> GATGRTTIAIDPVTRIEGHLKAEVVVENGKVVDARLSGGMYRGFETILRGRDPRDASQIVQRICGVCPTAHSTASVLALDEAFGAKVPNNGRITRNLIFGANYLQSHILHFYHLSAQDFVQGPDTAPFVPRFPKSDLRLSKELNKAGVDQYIEALEVRRICHEMVALFGGRMPHVQGQVVGGATEIPTKEKLVEYAARFKKVRDFVEQKYVPVVYTIGSKYKDMFKVGQGFKAALCVGAFPLDN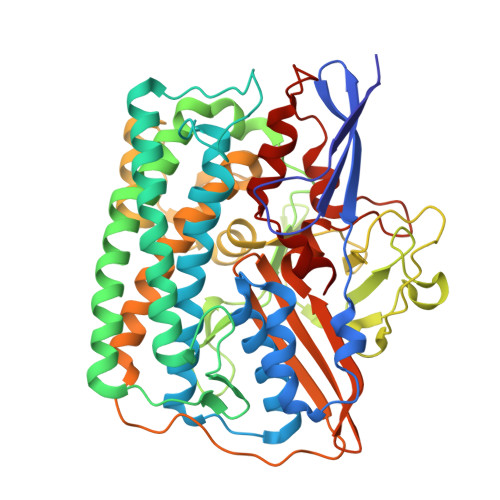SGKKHLFMPGVYAKGKDMPFDPSKIKEYVKYSWFAEETTGLNYKEGKTIPAPDKAGAYSFVKAPRYDGLSLEVGPLARMWVNNPELSPVGKKLLKDLFGISAKKFRDLGEEAAFSLMGRHVARAEETYYMLGAIEGWLKEIKAGEDTVVMPAVPASAEGTGFTEAPRGSLLHYVKVKDSKIDNYQIVSASLWNCNPRDDMGQRGAVEEALIGIPVDDIQNPVNVARLIRAFDPULACAVH> SPTVEECGYSDRVRSITLGNSTITTQECANVVVGYGRWPTYLRDDEATAEDQPTQPDVATCRFYTLDSIKWEKGSVGWWWKFPEALSDMGLFGQNMQYHYLGRAGYTIHVQCNASKFHQGCLLVVCVPEAEMGGAVVGQAFSATAMANGDKAYEFTSATQSDQTKVQTAIHNAGMGVGVGNLTIYPHQWINLRTNNSATIVMPYINSVPMDNMFRHY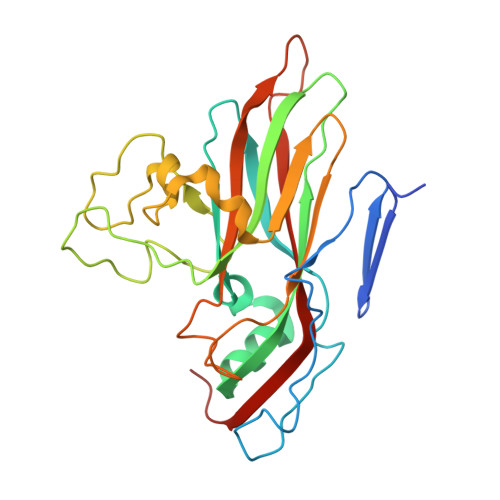NFTLMVIPFVKLDYADTASTYVPITVTVAPMCAEYNGLRLAQAQ4-{[(7R)-8-cyclopentyl-7-ethyl-5-methyl-6-oxo-5,6,7,8-tetrahydropteridin-2-yl]amino}-3-methoxy-N-(1-methylpiperidin-4-yl)benzamide 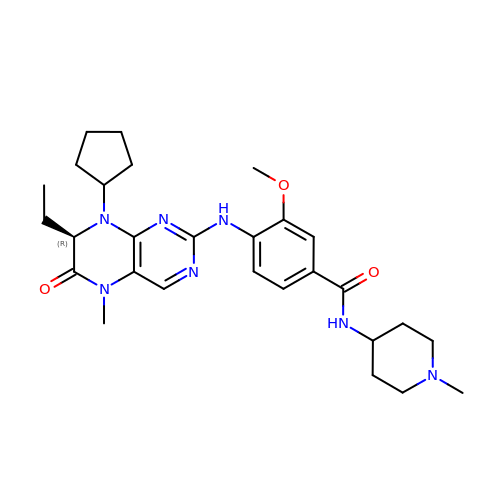| C28 H39 N7 O3 | XQVVPGYIWAGRNI-JOCHJYFZSA-N> MEGSEPVAAHQGEEASCSSWGTGSTNKNLPIMSTASVEIDDALYSRQRYVLGDTAMQKMAKSHVFLSGMGGLGLEIAKNLVLAGIKAVTIHDTEKCQAWDLGTNFFLSEDDVVNKRNRAEAVLKHIAELNPYVHVTSSSVPFNETTDLSFLDKYQCVVLTEMKLPLQKKINDFCRSQCPPIKFISADVHGIWSRLFCDFGDEFEVLDTTGEEPKEIFISNITQANPGIVTCLENHPHKLETGQFLTFREINGMTGLNGSIQQITVISPFSFSIGDTTELEPYLHGGIAVQVKTPKTVFFESLERQLKHPKCLIVDFSNPEAPLEIHTAMLALDQFQEKYSRKPNVGCQQDSEELLKLATSISETLEEKPDVNADIVHWLSWTAQGFLSPLAAAVGGVASQEVLKAVTGKFSPLCQWLYLEAADIVESLGKPECEEFLPRGDRYDALRACI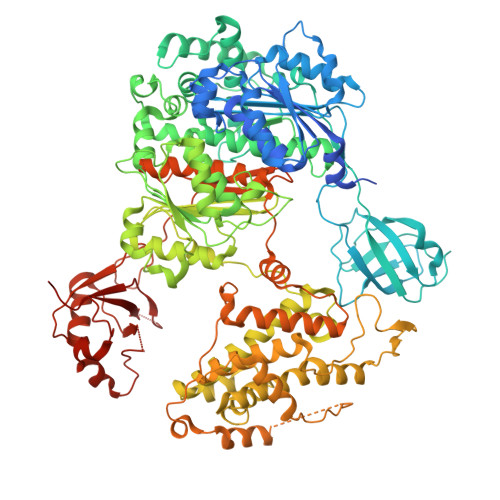GDTLCQKLQNLNIFLVGCGAIGCEMLKNFALLGVGTSKEKGMITVTDPDLIEKSNLNRQFLFRPHHIQKPKSYTAADATLKINSQIKIDAHLNKVCPTTETIYNDEFYTKQDVIITALDNVEARRYVDSRCLANLRPLLDSGTMGTKGHTEVIVPHLTESYNSHRDPPEEEIPIATLKNFPNAIEHTLQWARDEFEGLFKQPAENVNQYLTDPKFVERTLRLAGTQPLEVLEAVQRSLVLQRPQTWADCVTWACHHWHTQYSNNIRQLLHNFPPDQLTSSGAPFWSGPKRCPHPLTFDVNNPLHLDYVMAAANLFAQTYGLTGSQDRAAVATFLQSVQVPEFTPKSGVKIHVSDQELQSANASVDDSRLEELKATLPSPDKLPGFKMYPIDFEKDDDSNFHMDFIVAASNLRAENYDIPSADRHKSKLIAGKIIPAIATTTATVSGLVALEMIKVTGGYPFEAYKNCFLNLAIPIVVFTETTEVRKTKIRNGISFTIWDRWTVHGKEDFTLLDFINAVKEKYGIEPTMVVQGVKMLYVPVMPGHAKRLKLTMHKLVKPTTEKKYVDLTVSFAPDIDGDEDLPGPPVRYYFSHDTD> PPARKEKTKVKESVSRVEKAKQKSAQQELKQRQRAEIYALNRVMTE;> MDE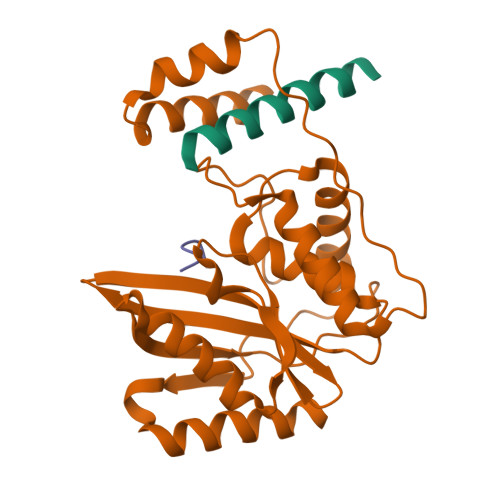ATWERMWKHVAKIHPDGEKVAQRIRGATDLPKIPIPSVPTFQPSTPVPERLEAVQRYIRELQYNHTGTQFFEIKKSRPLTGLMDLAKEMTKEALPIKCLEAVILGIYLTNSMPTLERFPISFKTYFSGNYFRHIVLGVNFAGRYGALGMSRREDLMYKPPAFRTLSELVLDFEAAYGRCWHVLKKVKLGQSVSHDPHSVEQIEWKHSVLDVERLGRDDFRKELERHARDMRLKIG;> GEEEGECY>[4x]GMSAGKTVVIALGGNAMLQAKEKGDYDTQRKNVEIAASEIYKIHKAGYKVVLTSGNGPQVGAIKLQNQAAAGVSPEMPLHVCGAMSQGFIGYMMSQAMDNVFCANNEPANCVTCVTQTLVDPKDQAFTNPTKPVGRFYTEQEAKDLMAA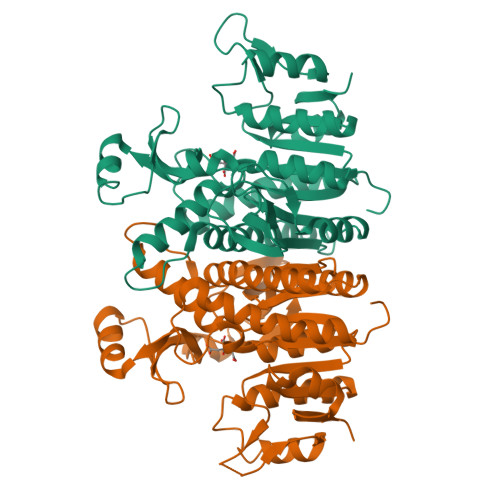NPGKILREDAGRGWRVVVPSPRPLEIVEYGVIKTLIDNNVLVICTNGGGIPCKRENKVISGVDAVIDKDLATSLLAKTLNSDYLMILTDVLNACINYKKPDERKLEEIKLSEILALEKDGHFAAGSMGPKVRAAIEFTQATGKMSIITSLSTAVDALNGKCGTRIIKD The replicative DNA pol from bacteriophage RB69 (RB69pol) is a member of the B family and is responsible for DNA synthesis of both leading and lagging strands of its genome. It has extensive sequence similarity to human replicative pols α and δ and therefore has been regarded as a good model for B family pols. Our previous reported 1.8 Å resolution structure of wt RB69pol showed that L415 is located right below the triphosphate tail of the incoming dNTP, where a small hydrophobic cavity exists at the tip of the L415 side chain. To provide a structural basis that could account for the different kinetic behavior observed among L415 variants and wt RB69pol, we determined the crystal structures of three ternary complexes: dTTP/dA-with the L415A mutant; dATP/dT-with the L415G mutant and dATP/dT-with the L415M mutant with resolutions ranging from 1.80 to 2.04 Å and Rfree values ranging from 21.3% to 21.9%.

Replacing L415 with either Ala or Gly greatly enlarges the size of this cavity. Similar differences were observed between structures of the L415G ternary complex and the wt RB69pol ternary complex. In particular, the change of the metal ion A position in both the L415A and L415G ternary complexes are mediated by an alteration in peptide backbone. The only discrepancy is that the backbones of T622 and S624 in the L415G ternary complex did not shift away from the position observed in wt RB69pol, instead the carboxyl group of D623 titled toward the cavity generated by the L415 to Gly substitution. For example, the L415G mutant has the largest cavity; thus, the corresponding side chains of L412 and D623 show the greatest tilt toward the cavity. In addition, a water molecule is observed in this hydrophobic cavity when L415 is replaced with Ala or Gly. In accord with these studies, this trapped water molecule is hydrogen bonded to both the carbonyl oxygen of T622 and G590. Therefore, the 0.5 Å downshifting of the metal ion A from its optimal position observed in the wt RB69pol structure would cause misalignment between the 3′-OH and Pα, possibly reducing the rate of phosphodiester bond formation. This could explain why the kpol values for incorporating a correct dNMP by L415A and L415G mutants are 5- to 25-fold lower than the kpol for wt RB69pol. Therefore, the FRET values for both P/Ts in the presence of the L415G mutant are not distinguishable so it appears that the L415G mutant cannot distinguish the control P/T from the Mis-P/T. Interestingly, the L415A mutant follows the same pattern.

> MKEFYLTVEQIGDSIFERYIDSNGRERTREVEYKPSLFAHCPESQATKYFDIYGKPCTRKLFANMRDASQWIKRMEDIGLEALGMDDFKLAYLSDTYNYEIKYDHTKIRVANFDIEVTSPDGFPEPSQAKHPIDAITHYDSIDDRFYVFDLLNSPYGNVEEWSIEIAAKLQEQGGDEVPSEIIDKIIYMPFDNEKELLMEYLNFWQQKTPVILTGWNVESFAIPYVYNRIKNIFGESTAKRLSPHRKTRVKVIENMYGSREIITLFGISVLDYIDLYKKFSFTNQPSYSLDYISEFELNVGKLKYDGPISKLRESNHQRYISYNIIAVYRVLQIDAKRQFINLSLDMGYYAKIQIQSVFSPIKTWDAIIFNSLKEQNKVIPQGRSHPVQPYPGAFVKEPIPNRYKYVMSFDLTSGYPSIIRQVNISPETIAGTFKVAPLHDYINAVAERPSDVYSCSPNGMMYYKDRDGVVPTEITKVFNQRKEHKGYMLAAQRNGEIIKEALHNPNLSVDEPLDVDYRFDFSDEIKEKIKKLSAKSLNEMLFRAQRTEVAGMTAQINRKLLINSLYGALGNVWFRYYDLRNATAITTFGQMALQWIERKVNEYLNEVCGTEGEAFVLYGDTDSIYVSADKIIDKVGESKFRDTNHWVDFLDKFARERMEPAIDRGFREMCEYMNNKQHLMFMDREAIAGPPLGSKGIGGFWTGKKRYALNVWDMEGTRYAEPKLKIMGLETQKSSTPKAVQKALKECIRRMLQEGEESLQEYFKEFEKEFRQLNYISIASVSSANNIAKYDVGGFPGPKCPFHIRGILTYNRAIKGNIDAPQVVEGEKVYVLPLREGNPFGDKCIAWPSGTEITDLIKDDVLHWMDYTVLLEKTFIKPLEGFTSAAKLDYEKKASLFDMF>[6x]GPAMASEVLQKTRKINKTLQTSGGSSVSFDLLAGALGDVLSSNVYVVSAKGKVLGLHLNDVQDSSVIEDEYTKQKKFSDEYTQNVLKIDETLENLNGEKILEIFPEEHGRLQKYTTVVPILGSGQRLGTLVLSRYSNSFNDDDLVIAEYSATVVGLEIL

CodY is found in nearly all low G+C Gram-positive bacteria and is activated by binding of one of the branched-chain amino acids (BCAAs; isoleucine, leucine, valine) and, in most species, GTP. The CodY protein represses transcription of hundreds of genes and activates transcription of dozens of other genes in many Gram-positive species. The global regulator, CodY, is also a strong repressor of the tcdR gene, as well as an inhibitor of sporulation. The cGMP-specific phosphodiesterases- adenylyl cyclases-FhlA (GAF) domain of B. subtilis CodY (BsCodY) protein, formed by the N-terminal 155 residues, includes a loop of amino acid residues that interact with BCAAs; such binding induces a change in protein structure leading to increased affinity for CodY-binding sites.

The GAF domain sequences of C. difficile and B. subtilis CodY proteins (44% identity) are not nearly as similar as the C-terminal, DNA-binding domains (93% identity). The crystal structure of the GAF domain of CdCodY bound to isoleucine was solved by molecular replacement and refined against data extending to 1.7 Å resolution, as described in Supplementary Materials and Methods and S1 Table. The CdCodY GAF domain was found to consist of a central, five-stranded, anti-parallel β-pleated sheet (β3-β4-β5-β1-β2) onto the bottom face of which are packed two α-helices, α2 and α4. The N-terminal α1 helix protrudes strikingly away from the rest of the GAF domain in CdCodY. Although they differ in sequence, the tertiary structure of the CdCodY GAF domain is similar to that of the GAF domain of BsCodY; 120 Cα atoms can be superposed with a root mean squared positional displacement (rmsΔ) of 1.5 Å. In both CdCodY and BsCodY, the effector isoleucine is bound in a pocket on the face of the β-sheet that is distal to the long helices α2 and α5, but the positions and modes of isoleucine binding are quite different. The CdCodY binding site is formed by residues from strands β1 and β5 from the β-pleated sheet and from the β2-β3 and β3-β4 segments of the polypeptide, which embrace the ligand so that it is completely enclosed in the protein interior. The first of the carboxylate oxygens of isoleucine forms an ion-pairing interaction with the ε-NH3+ of K110 and a charge-dipole interaction with the side chain hydroxyl of S130, with the second carboxylate oxygen forming charge-dipole hydrogen bonds with the phenolic hydroxyl of Y42 and the side chain amide–NH2 of N40. Meanwhile the α-amino group of the ligand forms an ion-pairing interaction with the side chain carboxylate of E104 and charge-dipole interactions with the hydroxyl of the side chain of S62 and the main chain carbonyl of D60. The isobutyl side chain, which distinguishes BCAAs from other amino acids, projects into a pocket circumscribed by the aromatic side chains of Y42, F74 and F101, and the aliphatic portions of the side chains of S62, S130 and E104.(2R)-2-(2,3-dihydro-1,4-benzodioxin-6-yl)pyrrolidine 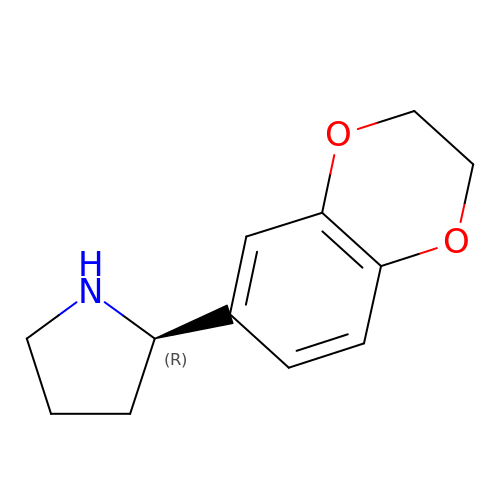| C12 H15 N O2 | LSNPFVDQLTUQCE-SNVBAGLBSA-N>[2x]MANFIEKITYLGTPAIKAGNEHLEMIVVPEWGSNVISLVDKTTNVQLLREPETAE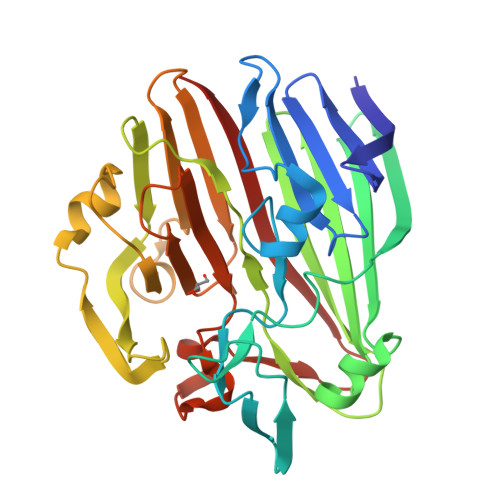SFHDTPTLYGIPILFPPNRISDGTFSFRGRTYHFDINEKDKHNHLHGFLYHEKWNVVTTKQTDEGVIVETEIDLSELPHVQKQFPHHAVVRMTYTIKENTLFKHATVMNKGKEAFPWGIGYHTTFIFPAESSLFSLTADQQWELDERLLPTGKLMDVPYKEALHEGMDLRHKQLDDVFLSSYQKRGGENQAVIYHQHAHISIIYKADEQFKHWVVYNADGKQGYLCPEPYTWVTNAVNLDLPSSLTGLQVLEPGEETTAKSSITIELNHQ>[6x]MTLYRLHEADLEIPDAWQDQSINIFKLPASGPAREASFVISRDASQGDAPFADYVARQLENAEKQLPGFKLH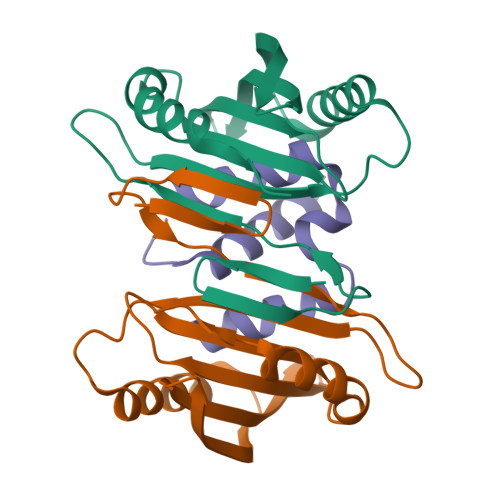KRWDINIHGHAAVLLDYQWQREGRDLMLRQVFIERRPAVLITTLTTTPADLPHHEPAWKQAMQTLVPRPTPSGS;>[3x]MDAQAAARLGDEIAHGFGVAAMVAGAVAGALIGAAVVAATAATGGLAAVILAGSIAAGGLSHHHHHH>GHMGVAVPHRAELARQLIDARNRTLRLVDFDDAELRRQYDPLMSPLVWDLAHIGQQEELWLLRGGDPRRPGLLEPAVEQLYDAFVHPRASRVHLPLLSPAQARRFCATVRSAVLDALDRLPEDADTFAFGMVVSHEHQHDETMLQALNLRSGEPLLGSGTALPPGRPGVAGTSVLVPGGPFVLGVDLADEPYALDNERPAHVVDVPAFRIGRVPVTNAEWRAFIDDGGYRQRRWWSDAGWAYRCEAGLTAPQFWNPDGTRTRFGHVEDIPPDEPVQHVTYFEAEAYA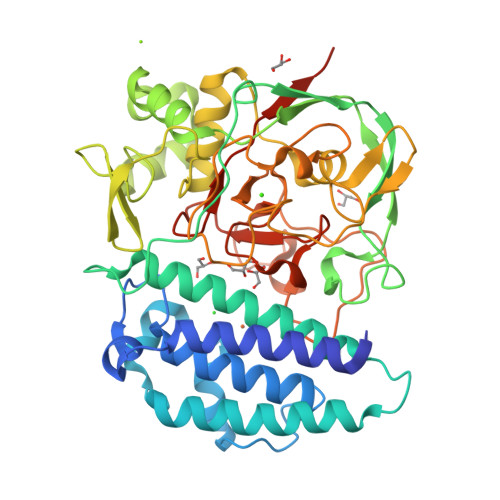AWAGARLPTEIEWEKACAWDPATGRRRRYPWGDAAPTAALANLGGDALRPAPVGAYPAGASACGAEQMLGDVWEWTSSPLRPWPGFTPMIYQRYSQPFFEGAGSGDYRVLRGGSWAVAADILRPSFRNWDHPIRRQIFAGVRLAWDVDRQTARPGPVGGC[2x]>GTNTGGVLVITDTIIVKSGQTYDGKGIKIIAQGMGDGSQSENQKPIFKLEKGANLKNVIIGAPGCDGIHCYGDNVVENVVWEDVGEDALTVKSEGVVEVIGGSAKEAADKVFQLNAPCTFKVKNFTATNIGKLVRQNGNTTFKVVIYLEDVTLNN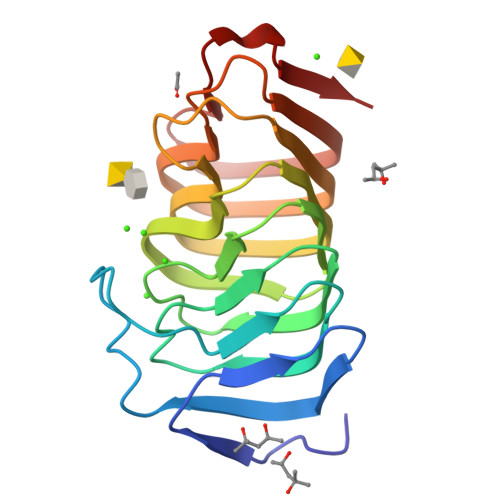VKSCVAKSDSPVSELWYHNLNVNNCKTLFEFPSQSQIHQY[2x]>MSALFEPYTLKDVTLRNRIAIPPMCQYMAEDGLINDWHQVHYASMARGGAGLLVVEATAVAPEGRITPGCAGIWSDAHAQAFVPVVQAIKAAGSVPGIQIAHAGRKASANRPWEGDDHIGADDARGWETIAPSAIAFGAHLPNVPRAMTLDDIARVKQDFVDAARRARDAGFEWIELHFAHGFLGQSFFSEHSNKRTDAYGGSFDNRSRFLLETLAAVREVWPENLPLTARFGVLEYDGRDEQTLEESIELARRFKAGGLDLLSVSVGFTIPETNIPWGPAFMGPIAERVRREAKLPVTSAWGFGTPQLAEAALQANQLDLVSVGRAHLADPHWAYFAAKELGVEKASWTLPAPYAHWLERYRLEHHHHHH[2x]

The biocatalytic reduction of the oxime moiety to the corresponding amine group has only recently been found to be a promiscuous activity of ene-reductases transforming α-oximo β-keto esters. By studying the crystal structures of enzyme oxime complexes, analyzing molecular dynamics simulations, and investigating biocatalytic cascades and possible intermediates, we obtained evidence that the reaction proceeds via an imine intermediate and not via the hydroxylamine intermediate. To gain more insight into the reaction pathway, we determined the crystal structures of the two enzymes OPR3 and XenA in complex with the oxime substrates 1a–c, either by co-crystallization or by soaking. All the crystal structures obtained had a high resolution (1.9–1.35 Å) and showed clear electron density features for the oximes.

To assess if the introduced amino acid exchanges affected the overall structure and the binding of the oxime, we also crystallized the tyrosine variants in complex with selected oxime substrates. The protomers in the crystal structures of the tyrosine variants are perfectly superimposable with the ones of the wild-type enzymes, confirming that the exchanges did not lead to major structural alterations. Interestingly, the binding mode of the oxime substrates also did not change in most of the structures. The propanoyl moiety of oxime 1b points into this cavity and is likely stabilized by hydrophobic interactions. Substrates with an acetyl moiety (such as oximes 1a and 1c) give the non-productive binding mode described above. Tyrosine 183, the canonical proton donor of XenA,55 is also found at a hydrogen bond distance from the Cα of the oxime. Looking at the results obtained for XenA, product formation was comparable for both tyrosine variants, the canonical Y183F and the non-canonical one (Y27F). The calculated high Kd for oxime 1b clearly indicates this enzyme’s low affinity for the substrate and might explain why this enzyme performed poorly in the biotransformation of the other oximes in our previous work. Both the Y183F and the Y27F variants of XenA showed a non-Michaelis–Menten behavior, with a linear increase of the rate over the concentration (bottom right).> KGNNCLDAAKACNLDDTCKKYRSAYITPCTTSMSNEVCNRRKCHKALRQFFDKVPAKHSYGMLFCSCRDIACTERRRQTIVPVCSYEERERPNCLSLQDSCKTNYICRSRLADFFTNCQPESRSVSNCLKENYADCLLAYSGLIGTVMTPNYVD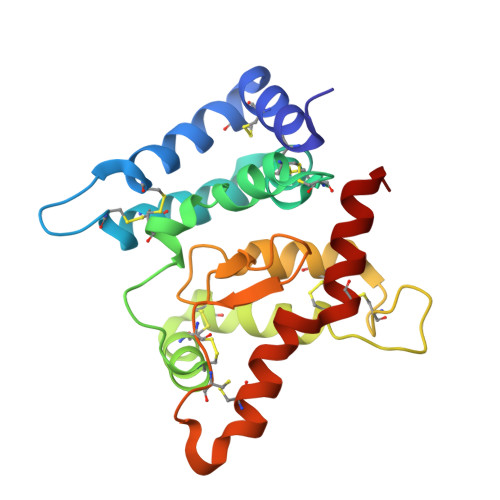SSSLSVAPWCDCSNSGNDLEDCLKFLNFFKDNTCLKNAIQAFGNGS> SHMFVNKDQIAKDVKQFYDQALQQAVVDDDANNAKAVVKTFHETVDCCGSSTLAALTTSVLKNNLCPSGSNIISNLLKKDCHQKIDDFFS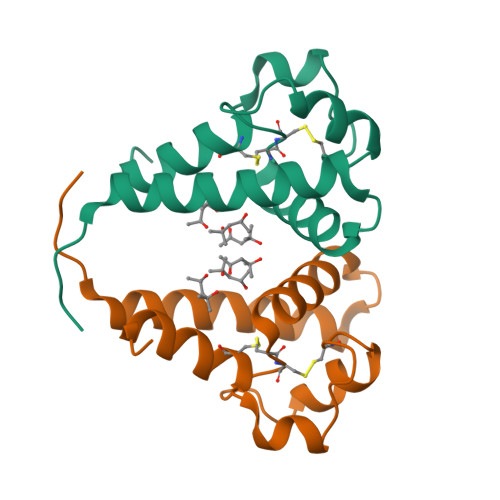GKL> AGQGDGSVIELGEQTVVATAQEETKQAPGVSIITAEDIAKRPPSNDLSQIIRTMPGVNLTGNSSSGQRGNNRQIDIRGMGPENTLILVDGKPVSSRNSVRYGWRGERDSRGDTNWVPADQVERIEVIRGPAAARYGNGAAGGVVNIITKQAGAETHGNLSVYSNFPQHKAEGASERMSFGLNGPLTENLSYRVYGNIAKTDSDDWDINAGHESNRTGKQAGTLPA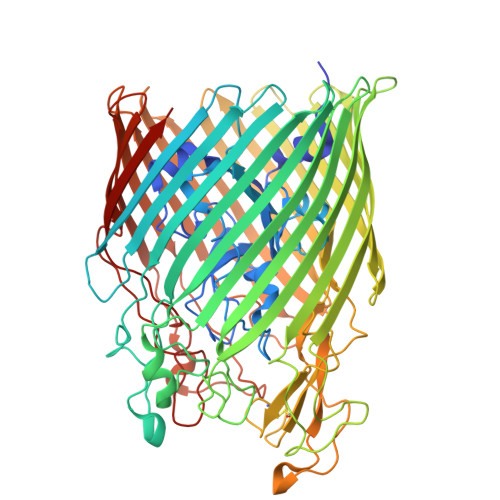GREGVRNKDIDGLLSWRLTPEQTLEFEAGFSRQGNIYTGDTQNTNSNNYVKQMLGHETNRMYRETYSVTHRGEWDFGSSLAYLQYEKTRNSRINEGLAVGTEGIFDPNNAGFYTATLRDLTAHGEVNLPLHLGYEQTLTLGSEWTEQKLDDPSSNTQNTEEGGSIPGLAGKNRSSSSSARIFSLFAEDNIELMPGTMLTPGLRWDHHDIVGDNWSPSLNLSHALTERVTLKAGIARAYKAPNLYQLNPDYLLYSRGQGCYGQSTSCYLRGNDGLKAETSVNKELGIEYSHDGLVAGLTYFRNDYKNKIESGLSPVDHASGGKGDYANAAIYQWENVPKAVVEGLEGTLTLPLADGLKWSNNLTYMLQSKNKETGDVLSVTPRYTLNSMLDWQATDDLSLQATVTWYGKQKPKKYDYHGDRVTGSANDQLSPYAIAGLGGTYRLSKNLSLGAGVDNLFDKRLFRAGNAQGVVGIDGAGAATYNEPGRTFYTSLTASF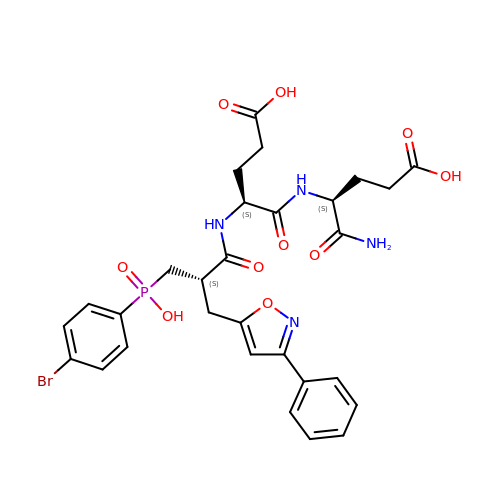N-{(2S)-3-[(S)-(4-bromophenyl)(hydroxy)phosphoryl]-2-[(3-phenyl-1,2-oxazol-5-yl)methyl]propanoyl}-L-alpha-glutamyl-L-alpha-glutamine | C29 H32 Br N4 O10 P | RXBMEHOLQJITJI-LEOXJPRUSA-N> MRMFRITACVPSQTRIRTQRELQNTYFTKLVPY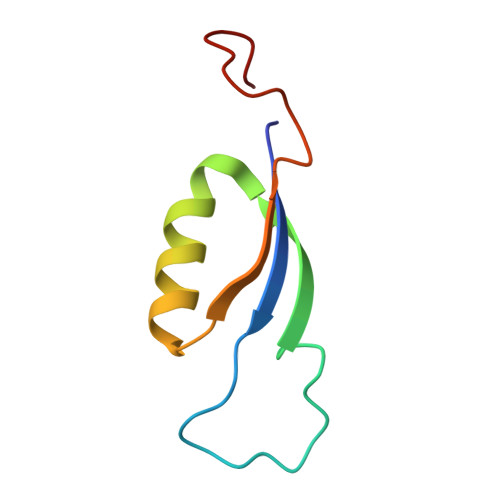DNWFREQQRIMKMGGKIVKVELATGRPGTNAGLA> MSLPEILPLEVIDKTINQKVLIVLQSNREFEGTLVGFDDFVNVILEDAVEWLIDPEDESRNEKVMQHHGRMLLSGNNIA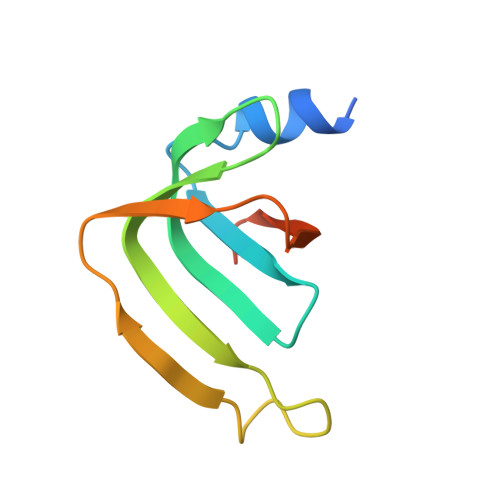ILVPGGKKTPTEAL>VRKGNKKLAKQATTKAVNPQPRRRNNNRRRGMRADAPLAKASTITGFGRGTNDVHLTGMSRIAQAVIPAGTGTDGYIVVDETIVPELLPRLGFAARIFQRYAVETLEFEIQPMCPANTGGGYVAGFLPDPTDSDHTFDAIQATRGAVVAKWWESRTIRPQYARALLWTSVGKEQRLTSPGRLILLCVGNNTDVVNVSVLCRWSVRLSVPSLETPEDTFAPILTLGPLYNDSLAANDFKSILLGSTQLDIAPEGAVYSLDRPLSIDYNLGTGDVDRAVYWHVKKVAGNAGTPAGWFHWGLWDNFNKTFTQGTAYYS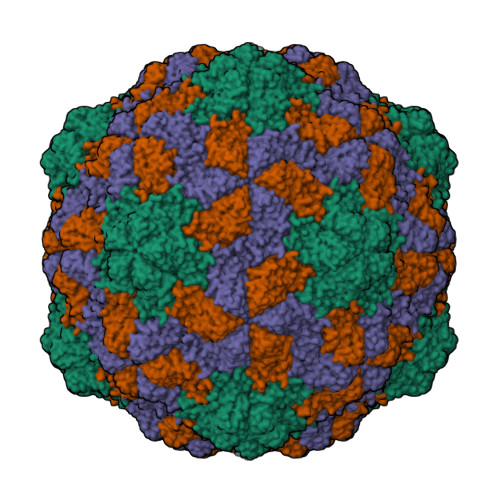DAQPRQILLPVGTLFTRADSGN[3x]>[2x]MMTGTIETTGNISAEKGGSIILQCHLSSTTAQVTQVNWEQQDQLLAICNA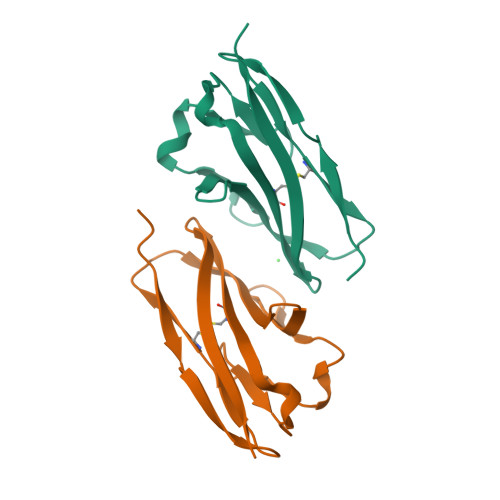DLGWHISPSFKDRVAPGPGLGLTLQSLTVNDTGEYFCIYHTYPDGTYTGRIFLEVLESSVAEHGAR>MKLAILGAGCYRTHAASGITNFSRACEVAEMVGKPEIAMTHSTITMGAELKELAGVDEVVVADPVFDNQFTVIDDFAYEDVIEAHKEDPEKIMPQIREKVNEVAKELPKPPEGAIHFTHPEDLGFEITTDDREAVADADFIMTWFPKGDMQPDIINKFIDDIKPGAIVTHACTIPTTKFYKIFEQKHGDLVTKPETLNVTSYHPGAVPEMKGQVYIAEGYASEDAIETLFELGQKARGNAYRLPAELLGPVCDMCSALTAITYAGILSYRDSVTQVLGAPASFAQMMAKESLEQITA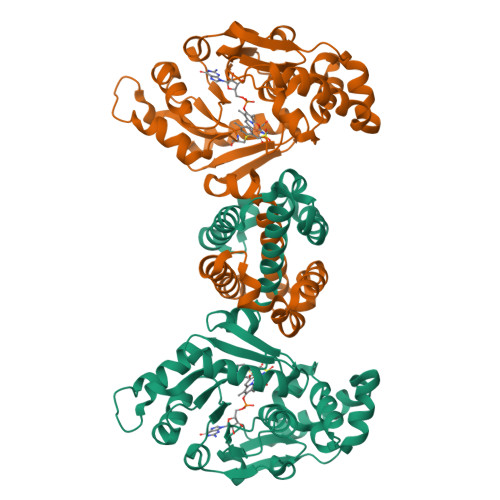LMEKVGIDKMEENLDPGALLGTADSMNFGASAEILPTVFEILEKRKK[2x]>AAIVPTRELENVFLGRCKDYEITRYLDILPRVRSDCSALWKDFFKAFSFKNPCDLDLGSYKDFFTSAQQQLPKNKVMFWSGVYDEAHDYANTGRKYITLEDTLPGYMLNSLVWCGQRANPGFNEKVCPDFKTCPVQARESFWGMASSSYAHSAEGEVTYMVDGSNPKVPAYRPDSFFGKYELPNLTNKVTRVKVIVLHRLGEKIIEKCGAGSLLDLEKLVKAKHFAFDCVE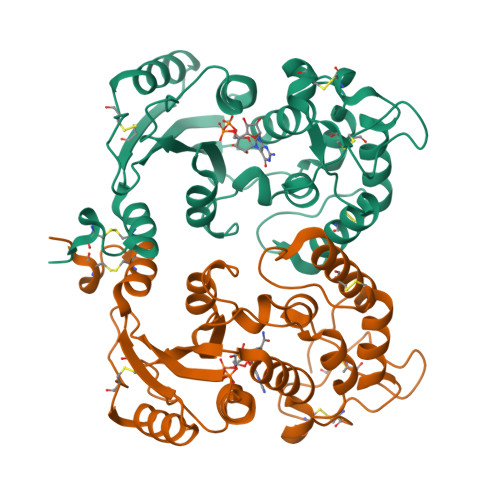NPRAVLFLLCSDNPNARECRLAKRFYRIA[2x]>GPGSEFRPQPLPPGWERRVDDRRRVYYVDHNTRTTTWQRPTMESVRNFEQWQSQRNQLQGAMQQFNQRYLYSASMLAAENDPYGPLPPGWEKRVDSTDRVYFVNHNTKTTQWEDPRTQGLQNEEPLPEGWEIRYTREGVRYFVDHNTRTTTFKDPRNGKSSVTKGGPQIAYERGFRWKLAHFRYLCQSNALPSHVKINVSRQTLFEDSFQQIMALKPYDLRRRLYVIFRGEEGLDYGGLAREWFFLLSHEVLNPMYCLFEYAGKNNYCLQINPASTINPDHLSYFCFIGRFIAMALFHGKFIDTGFSLPFYKRMLSKKLTIKDLESIDTEFYNSLIWIRDNNIEECGLEMYFSVDMEILGKVTSHDLKLGGSNILVTEENKDEYIGLMTEWRFSRGVQEQTKAFLDGFNEVVPLQWLQYFDEKELEVMLCGMQEVDLADWQRNTVYRHYTRNSKQIIWFWQFVKETDNEVRMRLLQFVTGTCRLPLGGFAELMGSNGPQKFCIEKVGKDTWLPRSHTCFNRLDLPPYKSYEQLKEKLLFAIEETEGFGQE[2x]

The HECT E3 ubiquitin ligases 1 (WWP1) and 2 (WWP2) are responsible for the ubiquitin-mediated degradation of key tumour suppressor proteins and are dysregulated in various cancers and diseases. Two members of the NEDD4 family, WW domain-containing E3 ligase 1 (WWP1) and 2 (WWP2), are of particular interest due to their targeting of the tumour suppressor protein phosphatase and tensin homolog (PTEN) as well as various other tumour suppressors and transcription factors. The HECT-E3 ligases may offer the best druggability as they participate directly in the Ub transfer, unlike the RING-type, and with their catalytic function relying on a single active-site cysteine. We evaluate their structure-activity relationship (SAR) by synthesis aided by molecular docking using X-ray crystal structures of WWP1 and WWP2 solved as part of this study and improved over those previously reported.

However, we were able to solve and refine structures for the apo-proteins which were improvements on previously published data. The available crystal structures for WWP1 (PDB ID: 6J1X20) and WWP2 (PDB ID: 5TJ819) have missing domains and/or high Rfree values. The WWP1-2L34H crystal structure was solved at a resolution of 3.17 Å in the previously unreported space group C2 with two molecules in the asymmetric unit. Interestingly, this is the most complete structure of WWP1 solved to date revealing a structured WW2 domain. The grid boxes to perform the docking simulations were generated in cavities on the HECT domain surrounding the active site cysteines 890 (WWP1) and 838 (WWP2) given the ability of NSC-217913 to interfere with ubiquitination. The ligand poses of compound 11 in both WWP1-2L34H and WWP2-LH are somewhat similar due to the similarities of the proposed binding site between these two enzymes. These poses show the imidazo[4,5-b]pyrazine moiety engaging in π-π interactions with the phenolic side chain of Tyr639WWP1-2L34H and Tyr587WWP2-LH alongside the Cys640WWP1-2L34H and Cys588WWP2-LH backbone amides participating in hydrogen bonding interactions with the imidazole nitrogen. However, the ethyl butyrate thioether chain interactions differ significantly between the two enzymes, most likely associated with the residue mutation at M865/I813. When docked against WWP1-2L34H, the side chain of 11 orients itself so as to interact with the guanidium ion of Arg855, orientating compound 11 in closer contact with Tyr639, allowing π-π interactions with both rings of the imidazo[4,5-b]pyrazine core. As the heterocycle is oriented very similarly in the predicted complexes with both WWP1-2L34H and WWP2-LH, it may be that the increased π-π interactions and ion-dipole interactions between the ester and guanidinium functionalities of 11 docked to WWP1-2L34H provide the additional strength of binding observed in the IC50 values.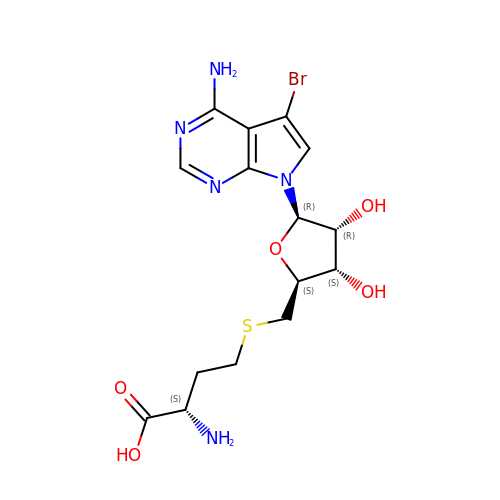(2S)-2-amino-4-({[(2S,3S,4R,5R)-5-(4-amino-5-bromo-7H-pyrrolo[2,3-d]pyrimidin-7-yl)-3,4-dihydroxytetrahydrofuran-2-yl]methyl}sulfanyl)butanoic acid (non-preferred name) | C15 H20 Br N5 O5 S | DIULHULFPSIBAK-TWBCTODHSA-N> GQKSDVIIGAEQTKAYFPILKNKRIAIFSNHTGMVGNKHLLDILLENNFNVVAIFSPEHGFRGNADAGEHVSSTIDSKTGVPILSLYNGKSKKPSEASMKKFDILIVDIQDVGLRFYTYYISMVRLMDACAEYDRKILILDRPNPNGHYVDGPILDMKYKSGVGGLPIPIVHGMTLGELALMVNGERWLPSSRICDVTVIPCKNYTHQTMYRLPIPPSPNLPNMKAIYLYPSICLFEGTPVSLGRGTTLPFQVYGHPNMTGYNYNFTPRSIPGAKNPPQLNKLCHGVNLSNLSDEEIWKKGINLDYLIDAYHNLNMGDRFFRPFFELLVGTDYVRKMIEGGKSADEIKARWKRDVERFKIQR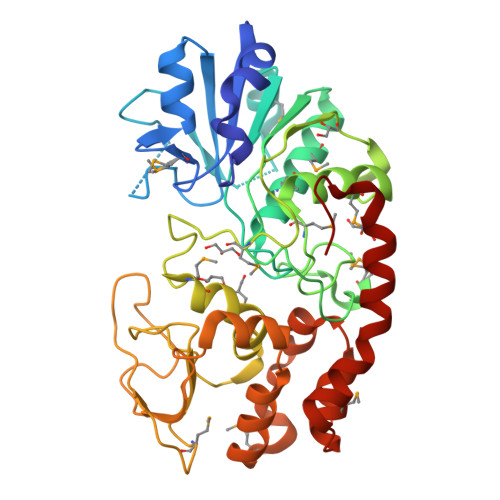KPYLLYQDN>MLIRRLKDARLRAGISQEKLGVLAGIDEASASARMNQYEKGKHAPDFEMANRLAKVLKIPVSYLYTPEDDLAQIILTWNELNEQERKRINFYIRKKAK[2x]

Controller proteins play a key role in the temporal regulation of gene expression in bacterial restriction–modification (R–M) systems and are important mediators of horizontal gene transfer. They form the basis of a highly cooperative, concentration-dependent genetic switch involved in both activation and repression of R–M genes. Here we present biophysical, biochemical, and high-resolution structural analysis of a novel class of controller proteins, exemplified by C.Csp231I. In contrast to all previously solved C-protein structures, each protein subunit has two extra helices at the C-terminus, which play a large part in maintaining the dimer interface.

The protein crystallised in two space groups: a monoclinic form (P21) and a cubic form (F4132). The calculated Matthews coefficients were 2.38 Å3 Da− 1 (one monomer in the asymmetric unit) and 2.01 Å3 Da− 1 (two monomers in the asymmetric unit) for the cubic and monoclinic structures, respectively. Thus, there is a crystallographic dyad between the two subunits in the cubic form, whereas the subunits are related by a noncrystallographic dyad in the monoclinic form. Structures from the two alternative space groups are very similar, and a least-squares fit of the monomer from the cubic unit cell data to either of the monomers from the monoclinic unit cell data gave an RMSD of 0.94 Å. A comparison of the dimers (formed by a crystallographic dyad in the cubic form and by a noncrystallographic dyad in the monoclinic form) resulted in an RMSD of 1.31 Å, reflecting a slight hinge movement at the dyad interface. A similar analysis of the monoclinic form of C.Csp231I reveals the same major features at the dimer interface, with an equivalent pair of interchain H-bonds. The buried surface area is reduced by ca 200 Å due to a small outward rotation of the final C-terminal helices relative to each other (residues 88–96), which may in part be due to the observed differences in crystal packing contacts in this region. The analysis of B-factors in the cubic crystal form of C.Csp231I reveals that the extended C-terminal region of the protein, comprising helices 6 and 7, is significantly more mobile than the rest of the structure. This is not so apparent in the monoclinic form, where crystal packing forces stabilise this region and the B-factors are more evenly distributed throughout the entire structure.> GSGPIDFWSSHPGQSSAAERELIGRFQDRFPTLSVKLIDAGKDYDEVAQKFNAALIGTDVPDVVLLDDRWWFHFALSGVLTALDDLFGQVGVDTTDYVDSLLADYEFNGRHYAVPYARSTPLFYYNKAAWQQAGLPDRGPQSWSEFDEWGPELQRVVGAGRSAHGWANADLIS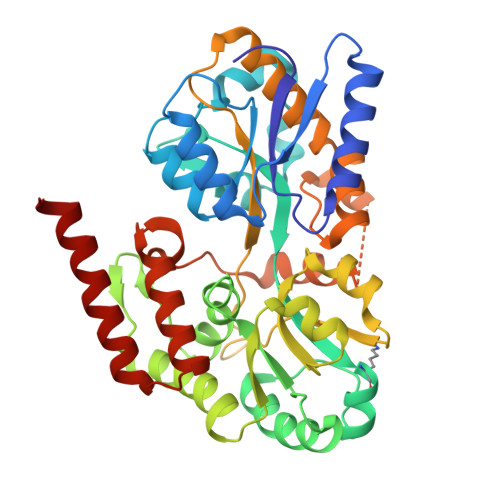WTFQGPNWAFGGAYSDKWTLTLTEPATIAAGNFYRNSIHGKGYAAVANDIANEFATGILASAVASTGSLAGITASARFDFGAAPLPTGPDAAPACPTGGAGLAIPAKLSEERKVNALKFIAFVTNPTNTAYFSQQTGYLPVRKSAVDRARVALDQLPHTRTQDYARVFLPGGDRIISAGLESIGLRGADVTKTFTNIQKRLQVILDRQIMR>[2x]LPEHVDWRAKGAVIPLKNQGKCGSCWAFSTVTTVESINQIRTGNLISLSEQQLVDCSKKNHGCKGGYFDRAY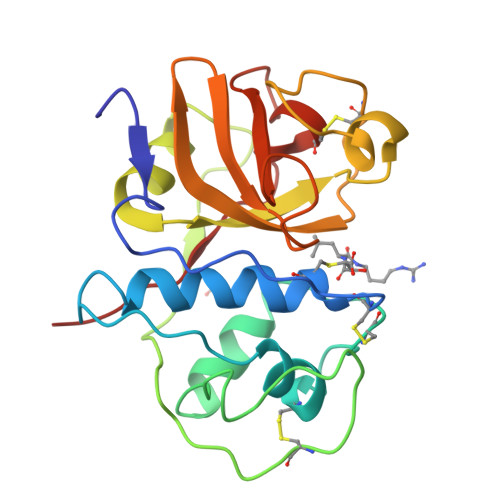QYIIANGGIDTEANYPYKAFQGPCRAAKKVVRIDGCKGVPQCNENALKNAVASQPSVVAIDASSKQFQHYKGGIFTGPCGTKLNHGVVIVGYGKDYWIVRNSWGRHWGEQGYTRMKRVGGCGLCGIARLPFYPTKAX> STHFRTFRSQADFSSITRASSLLDACGFYWGPLTVSAAHEKLKSEPEGTFLIRDSTQKNCFF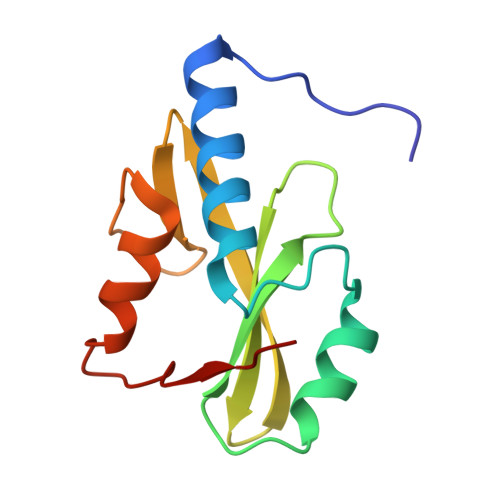AISVKTATGPTSIRINFQTGRFSLDGSKETFDCLFKLLEHYLSSPRKVLVTPLRK>[2x]NIMSSAFYQQIQQQIEEVKAEGLYKSERIITSQQQAAVKIASGEEVLNFCANNYLGLANHPALIEAGKAGMDEHGFGMASVRFICGTQDIHKELEQKLSTFLGKEDTILYTSCFDANAGLFETILDKEDAIISDALNHASIIDGVRLCKAMRFRYSNNNMTELEEQLIAAKDAGARNILIVTDGVFSMDGVVANLPAICDLAEKYGALTMVDDSHAVGFMGKTGAGTHEYHDVVDRIDIITGTLGKAMGG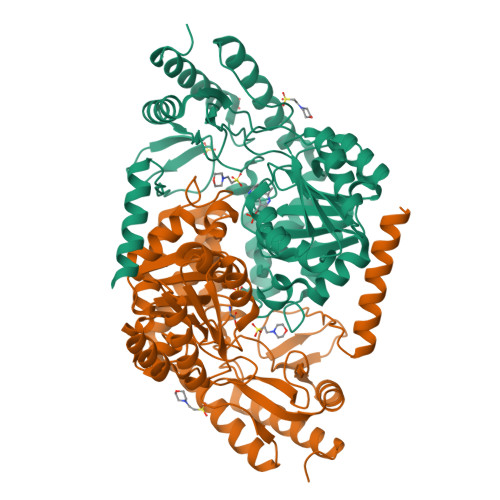ASGGYTSGKKEVIEWLRQRSRPYLFSNSVAPAIVSASIRVLDLLQESGDLRDRLWENATHFRTRMSEAGFTLAGADHAIIPIMLGDAKVAAEFAERALEKGIYVIGFSFPVVPKGQARIRTQMSAAHSREQLDKAIDAFIEVGRDMEIIK> MSKLTTGSFSIEDLESVQITINNIVGAAKEAAEEKEKELVNAGPTLFPGLEGYRDDWNFKLLDRYEPVITPMCDQCCYCTYGPCDLSGNKRGACGIDMKGHNGREFFLRVITGTACHAAHGRHLLDHLIEKYGEDLPLTLGQSNVLTPNITISTGLSPKTLGEVKPAMEYVEEQLTQLLATVHAGQESAEIDYDSKALFSGSLDHVGMEISDIVQVAAYDFPKADPEAPLVEIGMGTIDKSKPFLCVIGHNVAGVTYMMDYMEDNNLTDKMEIAGLCCTAIDLTRYKEADRRPPYAKVIGSMSKELKVIRSGMPDVIVVDEQCVRGDIVPEAQKLKIPVIASNPKIMYGLPNRTDADVDETMEELKSGKIPGCVMLDYDKLGELCVRLTMEMAPIRDAAGITALPTDEELVNMVAKCADCGACLLACPEEIDIPEAMGFAKKGDFSYFEEIHDTCIGCRRCEQVCKKEIPILNVIEKIAQKQIAEEKGLMRAGRGQVSDAEIRAEGLNLVMGTTPGIIAIIGCPNYAGGTKDVYYIAEEFLKR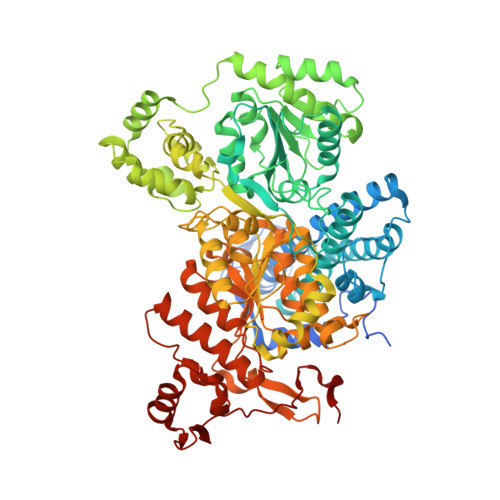NFIVVTTGCGAMDIGMFKDADGKTLYERFPGGFQCGGLANIGSCVSNAHITGAAEKVAAIFAQRTLEGNLAEIGDYILNRVGACGLAWGAFSQKASSIGTGCNIFGIPAVLGPHSSKYRRALIAKTYEEDKWKVYDARNGQEMPIPPAPEFLLTTAETWQEAIPMMAKACIRPSDNSMGRAIKLTHWMELHKKYLGGKEPEDWWKFVRTEADLPLATREALLKELEKEHGWEIDWKRKKIISGPKIKFDVSAQPTNLKRLCKEA>MAHHHHHHMSKPETTAAPNFLRQIVQADLDAGKHAKIVTRFPPEPNGYLHIGHAKSICLNFGLAQEFAGDCHLRFDDTNPAKEDQEYIDAIEADIKWLGFQWSGEVCYASNYFD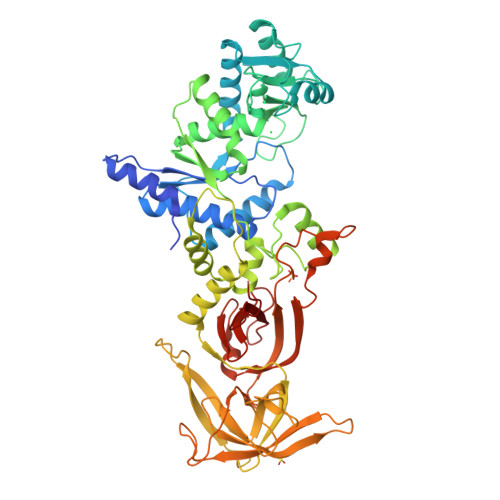QLHAWAVELIKAGKAFVCDLGPEEMREYRGTLTEPGRNSPYRDRSVEENLDLFARMKAGEFPDGARSLRAKIDMGSPNMNLRDPILYRIRHAHHHQTGDKWCIYPSYDFTHGQSDAIEGITHSICTLEFEDHRPLYEWFLANLPVPAQPRQYEFSRLNLNYTVTSKRKLKQLVDEGHVSGWDDPRMSTLSGYRRRGYTPESIRNFCEMIGVNRASGVVDIGMLEFSIRDHLDATAPRAMCVLKPLKVVITNYPEGQVENLELPRHPKEDMGVRVLPFGRELFIDAGDFEEVPPAGYKRLIPGGEVRLRGSYVIRADEAIKDADGNIVELRCSYDPDTLGKNPEGRKVKGVIHWVPAEGSVECEVRLYDRLFRSANPEKAEEGGSFLDNINADSLQVLAGCRAEPSLGQANPEDRFQFEREGYFVADLKDSRPGKPVFNRTVTLRDSWGQG[2x]>GSHMAHQPSDTIAGLYEAFNSGDLETLRELIA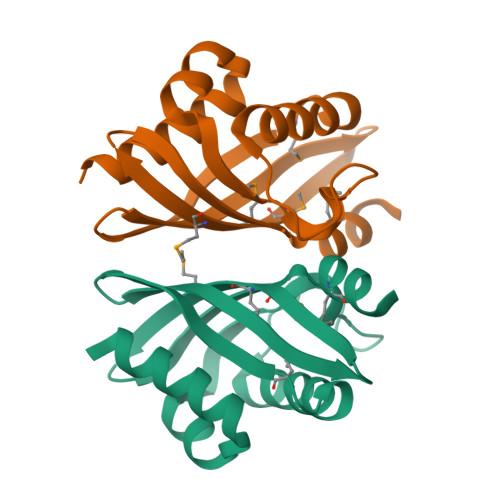PDAVIHLPGTAGDAEHPPGTPRDREGWLGVWQFTQAFFPDMTATVQDIVQTGDLVATRCVARGTHSGRPFEMTMLNMSRVRDGRIVEHWTISDNVTMLAQLGVKASL[2x]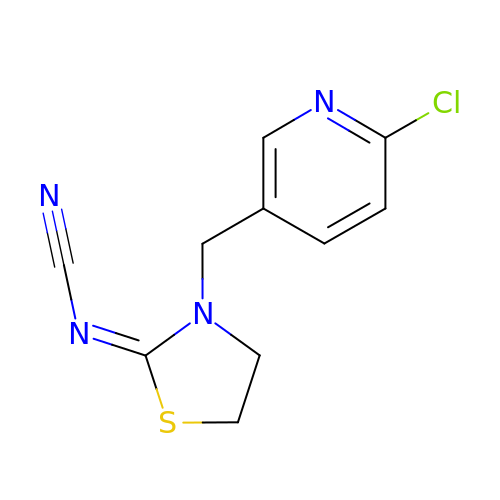{(2Z)-3-[(6-chloropyridin-3-yl)methyl]-1,3-thiazolidin-2-ylidene}cyanamide | C10 H9 Cl N4 S | HOKKPVIRMVDYPB-UVTDQMKNSA-N>[2x]STHFDVIVVGAGSMGMAAGYQLAKQGVKTLLVDAFDPPHTNGSHHGDTRIIRHAYGEGREYVPLALRSQELWYELEKETHHKIFTKTGVLVFGPKGESAFVAETMEAAKEHSLTVDLLEGDEINKRWPGITVPENYNAIFEPN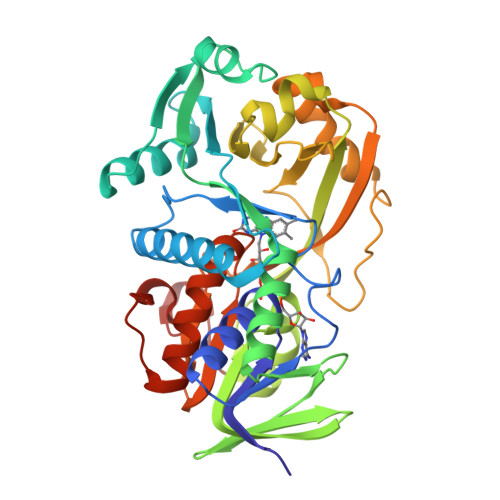SGVLFSENCIRAYRELAEARGAKVLTHTRVEDFDISPDSVKIETANGSYTADKLIVSMGAWNSKLLSKLNLDIPLQPYRQVVGFFESDESKYSNDIDFPGFMVEVPNGIYYGFPSFGGCGLMLGYHTFGQKIDPDTINREFGVYPEDESNLRAFLEEYMPGANGELKRGAVCMYTKTLDEHFIIDLHPEHSNVVIAAGFSGHGFKFSSGVGEVLSQLALTGKTEHDISIFSINRPALKESLQKTTI>[2x]SNATNSEKTNVYLANTVSTVTKKVSDIQSSKGLVYNENIPLFIN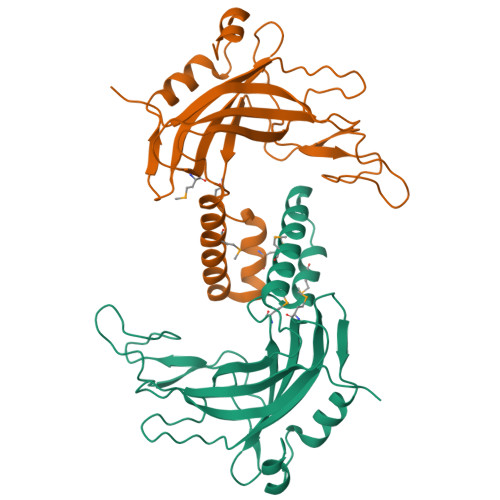NSKIQYDDTPYHWPSNVISLTNSSEKAIMDYEITCLAYDKNGKPLELYWDAQNVAADGEVGSVGFSPAGVDYGIVTGISPVSPKSYSHTYRKMQQSPPQDIISMFEKQQGKAWVENWLKEWKQMEKEYAKQNAIAPGKNQNDAFLLFDKWKQSTGEHGVKYIISCVKQVTFNDGSVWKNSAYENWLKSFQGKEVSNSVLENYYK> MASFIDLFAGDITTQLLKLLALVANTVYSCKGIAERLITMIRDVQPTIREIQYSGAELSNHHQTQLGVFYEILEKARKLCEKVLRCNRWNLKHVYHANKMKDLEKQISRFLNSQILLFVLAEVCHLRVNGDRIERNMDRLLTERNDSLSFPETMMEIETVSDPEIQTVLELGKKKVKEMMFKFTDTHLFGISGMSGSGKTTLAIELSKDDDVRGLFKNKVLFLTVSRSPNFENLESCIREFLYDGVHQRKLVILDDVWTRESLDRLMSKIRGSTTLVVSRSKLADPRTTYNVELLKKDEAMSLLCLCAFEQKSPPSPFNKYLVKQVVDECKGLPLSLKVLGASLKNKPERYWEGVVKRLLRGEAADETHESRVFAHMEESLENLDPKIRDCFLDMGAFPEDKKIPLDLLTSVWVERHDIDEETAFSFVLRLADKNLLTIVNNPRFGDVHIGYYDVFVTQHDVLRDLALHMSNRVDVNRRERLLMPKTEPVLPREWEKNKDEPFDAKIVSLHTGEMDEMNWFDMDLPKAEVLILNFSSDNYVLPPFIGKMSRLRVLVIINNGMSPARLHGFSIFANLAKLRSLWLKRVHVPELTSCTIPLKNLHKIHLIFCKVKNSFVQTSFDISKIFPSLSDLTIDHCDDLLELKSIFGITSLNSLSITNCPRILELPKNLSNVQSLERLRLYACPELISLPVEVCELPCLKYVDISQCVSLVSLPEKFGKLGSLEKIDMRECSLLGLPSSVAALVSLRHVICDEETSSMWEMVKKVVPELCIEVAKKCFTVDWLDD;> MAFEALTGINGDLITRSWSASKQAYLTERYHKEEAGAVVIFAFQPSFSEKDFFDPDNKSSFGEIKLNRVQFPCMRKIGKGDVATVNEAFLKNLEAIIDPRTSFQASVEMAVRSRKQIVFTGHSSGGATAILATVWYLEKYFIRNPNVYLEPRCVTFGAPLVGDSIFSHALGREKWSRFFVNFVSRFDIVPRIMLARKASVEETLPHVLAQLDPRKSSVQESEQRITEFYTRVMRDTSTVANQAVCELTGSAEAFLETLSSFLELSPYRPAGTFVFSTEKRLVAVNNSDAILQMLFYTSQASDEQEWSLIPFRSIRDHHSYEELVQSMGKKLFNHLDGENSIESTLNDLGVSTRGRQYVQAALEEEKKRVENQKKIIQVIEQERFLKKLAWIEDEYKPKCQAHKNGYYDSFKVSNEENDFKANVKRAELAGVFDEVLGLMKKCQLPDEFEGDIDWIKLATRYRRLVEPLDIANYHRHLKNEDTGPYMKRGRPTRYIYAQRGYEHYILKPNGMIAEDVFWNKVNGLNLGLQLEEIQETLKNSGSECGSCFWAEVEELKGKPYEEVEVRVKTLEGMLGEWITDGEVDDKEIFLEGSTFRKWWITLPKNHKSHSPLRDYMMDEITDT;> MDDCRFETSELQASVMISTPLFTDSWSSCNTANCNGSIKIHDIAGITYVAIPAVSMIQLGNLVGLPVTGDVLFPGLSSDEPLPMVDAAILKLFLQLKIKEGLELELLGKKLVVITGHSTGGALAAFTALWLLSQSSPPSFRVFCITFGSPLLGNQSLSTSISRSRLAHNFCHVVSIHDLVPRSSNEQFWPFGTYLFCSDKGGVCLDNAGSVRLMFNILNTTATQNTEEHQRYGHYVFTLSHMFLKSRSFLGGSIPDNSYQAGV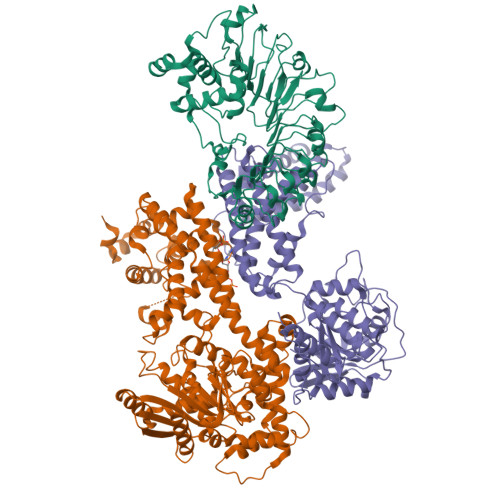ALAVEALGFSNDDTSGVLVKECIETATRIVRAPILRSAELANELASVLPARLEIQWYKDRCDASEEQLGYYDFFKRYSLKRDFKVNMSRIRLAKFWDTVIKMVETNELPFDFHLGKKWIYASQFYQLLAEPLDIANFYKNRDIKTGGHYLEGNRPKRYEVIDKWQKGVKVPEECVRSRYASTTQDTCFWAKLEQAKEWLDEARKESSDPQRRSLLREKIVPFESYANTLVTKKEVSLDVKAKNSSYSVWEANLKEFKCKMGYENEIEMVVDESDAMET> MPNRFVIADPKRCLGCYTCIAACAFVHEEQGLQPFPRLYLTYTSEGIMPIQCRHCEDAPCAEVCPVEAIKKEGNAIIIDEKACIGCKTCLLACSFGAIDFSVQDS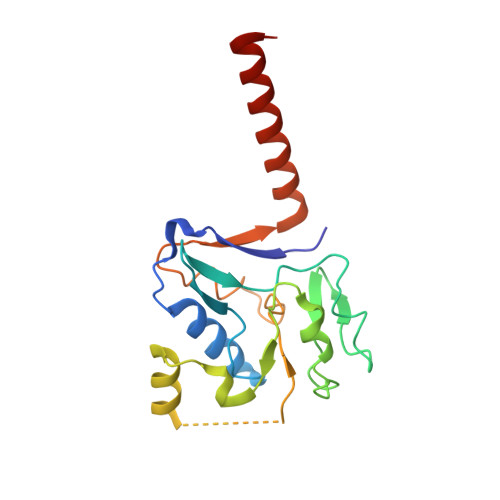LEQSIFKDIKENLMQDQKTQQRIVAVKCDLCNFREEGPACVQFCPTKALKLVDGDEINKMVKNKRTVNVESLLSVYGTK> MNNKEVELYGGAITTVVP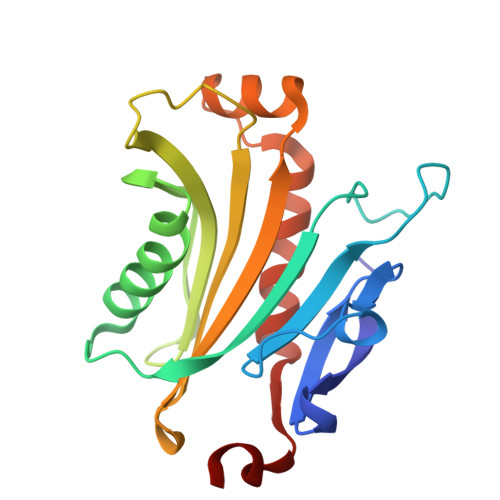PGFIDASTLREVPDTQAVYVNSRRDEEEFEDGLATNESIIVDLLETVDKSDLKEAWQFHVEDLTELNGTTKWEALQEDTVQQGTKFTGLVMEVANKWGKPDLAQTVVIGVALIRLTQFDTDVVISINVPLTKEEASQASNKELPARCHAVYQLLQEMVRKFHVVDTSLFA>[4x]HHHHHHGPNTNPVAAWKALKEGNERFVAGRPQHPSQSVDHRAGLAAGQKPTAVIFGCADSRVAAEIIFDQGLGDMFVVRTAGHVIDSAVLGSIEYAVTVLNVPLIVVLGHDSCGAVNAALA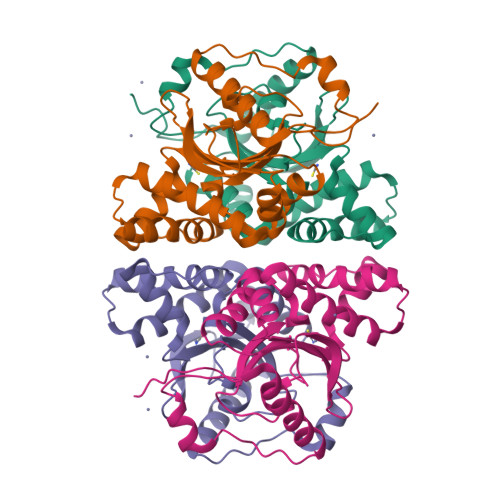AINDGTLPGGYVRDVVERVAPSVLLGRRDGLSRVDEFEQRHVHETVAILMARSSAISERIAGGSLAIVGVTYQLDDGRAVLRDHIGNIGEEV> EAEAEFANILPDIENEDFIKDCVRIHNKFRSEVKPTASDMLYMTWDPALAQIAKAWASNCQFSHNTRLKPPHKLHPNFTSLGENIWTGSVPIFSVSSAITNWYDEIQDYDFKTRICKKVCGHYTQVVWADSYKVGCAVQFCPKVSGFDALSNGAHFICNYGPGGNYPTWPYKRGATCSACPNNDKCLD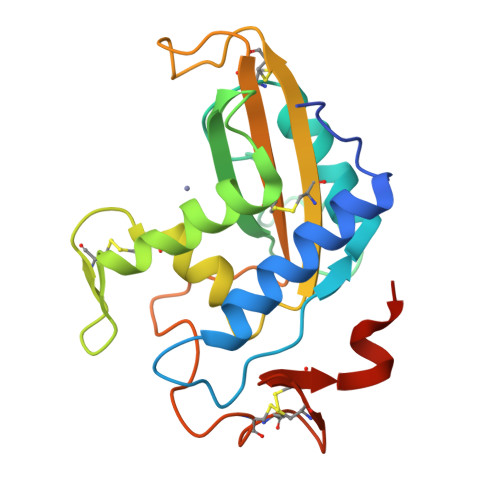NLCVNRQRDQVKRYYSV>HHHHHHSSGGMKALVYTGVAQLAFRDVPEPVPAAGDHLIRIDSVGICGSDMHAYLGHDDRRPAPLILGHEGAGVIIGGPRDGERVTINPLVTCGTCPACVSGRDNLCATRQIISMPPRDGAFAQYVAMPARNLVTVPDDVPLEKAALAEPVAVSWHAVRLGLASMADARRDSALVIGGGAIGVAAAISLQAQGVADVTLVEPNAMRREYLARDANYTIATPEQVAGRVFDITVDGVGYDATRAAASAATRPGGLLLHIGLGGGSAGLDIRRITLQEITVIGTYTYTAQDFRDTCAAMFDGRLGGLDWTESRPLSAGADAFADIRAGRVPAPKIILKP[4x]

Dihydroxypropanesulfonate (DHPS), a globally abundant organosulfur compound, serves as an ecologically important currency for nutrient and energy transfer from phytoplankton to bacteria in the ocean. A novel chiral-selective DHPS catabolic pathway was identified in marine Roseobacteraceae strains, where HpsO and HpsP dehydrogenases at the gateway to DHPS catabolism act specifically on R-DHPS and S-DHPS, respectively. R-DHPS is also a substrate for the dehydrogenase HpsN. All three dehydrogenases generate stable hydrogen bonds between the chirality-center hydroxyls of DHPS and highly conserved residues, and HpsP also form coordinate–covalent bonds between the chirality-center hydroxyls and Zn2+, which determines the mechanistic basis of strict stereoselectivity.

We solved the structure of DsHpsP from D. shibae DFL 12, which shared a substantial amino acid sequence identity (68%) with RpHpsP from R. pomeroyi DSS-3 and also possesses enantioselectivity for S-DHPS. The crystal structure of DsHpsP showed that four monomers, each containing two Zn2+ ions, constituted a tetramer in the asymmetric unit. DsHpsP is a member of the medium-chain alcohol dehydrogenases/reductase (MDR) superfamily, with a Rossmann-like fold domain for co-factor binding and a catalytic domain harboring essential catalytic residues and a metal atom. Loop 1 and loop 2 exhibited a rather constricted channel in the ligand-free state, but displayed an “open” state, with movement apart, upon binding of NAD+ and S-DHPS, suggesting a gating function for these loops in ligand entry. In the “open” state, the C3-OH of S-DHPS formed hydrogen-bonding interactions with His59, Glu60 and Glu139, as well as coordinate bonds with Zn2+. ICP-MS analysis revealed the presence of Zn2+ and Mn2+ in the protein. These results indicated that metals play an essential role in DsHpsP’s catalytic function. Site-directed mutagenesis suggested that His59 functions as the catalytic residue, as mutant His59Ala completely abolished the catalytic activity for S-DHPS. Glu60Ala and Glu139Ala displayed weak catalytic activities for S-DHPS, implying that Glu60 and Glu139 probably play roles in binding S-DHPS. The chirality-center C2-OH of S-DHPS could form a hydrogen bond with Glu139 and a coordinate bond with Zn2+, and these interactions disappeared when R-DHPS was replaced with S-DHPS at the active pocket, due to steric hindrance caused by the reverse chiral direction of C2-OH in R-DHPS. Moreover, the essential residues His59, Glu60, and Glu139 of DsHpsP from D. shibae DFL 12 were conserved in RpHpsP. Together, these suggest their common enzymatic functions and mechanisms, in which the interactions with C2-OH of S-DHPS determine the stereoselectivity of HpsP.> GPLGSGETVK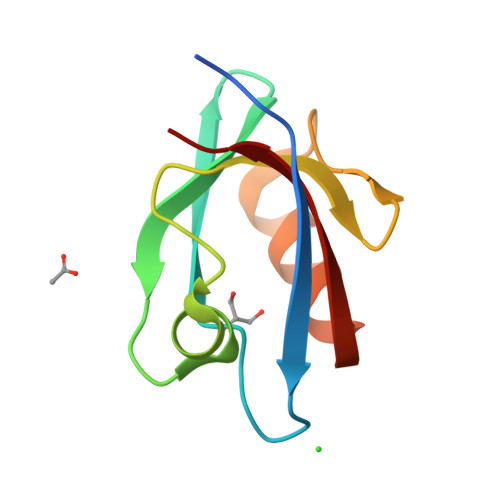IVRIEKARDIPLGATVRNEMDSVIISRIVKGGAAEKSGLLHEGDEVLEINGIEIRGKDVNEVFDLLSDMHGTLTFVLIPS> MNVQDRRRLLGPAAAKPMA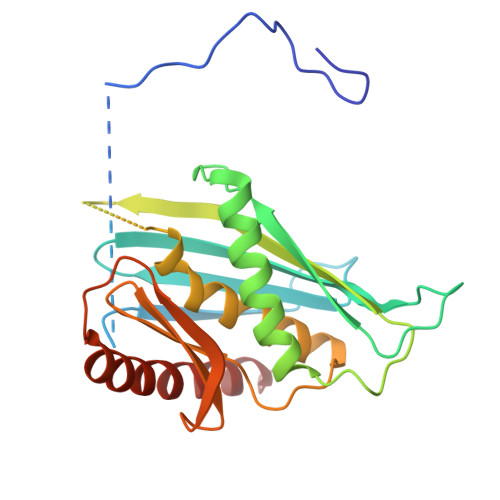FSNTTTHVPEKKSTDLTPKGNESEQELSLHTGFIENCNGSALVEARSLGHQTSLISAVYGPRSIRGSFTSQGTISIQLKNGLLEKYNTNELKEVSSFLMGIFNSVVNLSRYPKSGIDIFVYLTYDKDLTNNPQDDDSQSKMMSSQISSLIPHCITSITLALADAGIELVDMAGAGEANGTVVSFIKNGEEIVGFWKDDGDDEDLLECLDRCKEQYNRYRDLMISCLMNQET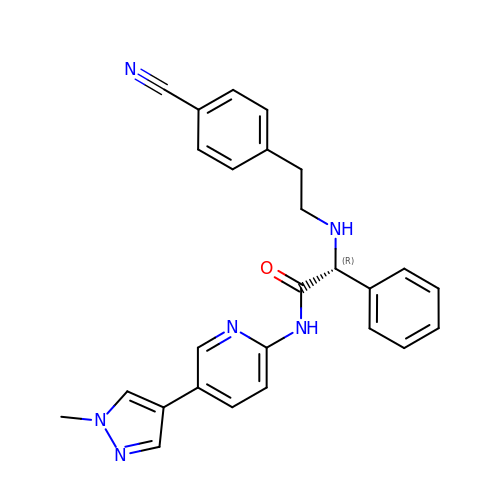(2R)-2-{[2-(4-cyanophenyl)ethyl]amino}-N-[5-(1-methyl-1H-pyrazol-4-yl)pyridin-2-yl]-2-phenylacetamide | C26 H24 N6 O | ZJGMOHOOSGHFMJ-RUZDIDTESA-N> MKNDYRTFKLSLLTLAPIHIGNGEKYTSREFIYENKKFYFPDMGKFYNKMVEKRLAEKFEAFLIQTRPNARNNRLISFLNDNRIAERSFGGYSISETGLESDRNPNSAGA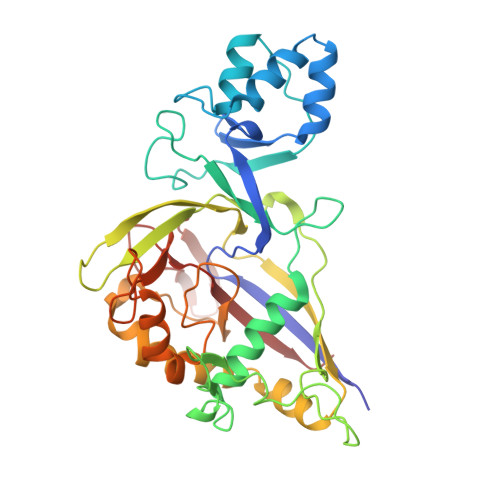INEVNKFIRDAFGNPYIPGSSLKGAIRTILMNTTPKWNNENAVNDFGRFPKENKNLIPWGPKKGKEYDDLFNAIRVSDSKPFDNKRLILVQKWDYSAKTNKAKPLPLYRESISPLTKIEFEITTTTDEAGRLIEELGKRAQAFYKDYKAFFLSEFPDDKIQANLQYPIYLGAGSGAWTKTLFKQADGILQRRYSRMKTKMVKKGVLKLTKAPLKIVKIPSGNHSLIKNHESFYEMGKANFMIKEIDK> XMHLNPAEKEKLQIFLASELLLRRKARGLKLNYPEAVAIITSFIMEGARDGKTVAMLMEEGKHVLTRDDVMEGVPEMIDDIQAEATFPDGTKLVTVHNPIS;> MSNNNYIVPGEYRVAEGEIEINAGREKTTIRVSNTGDRPIQVGSHIHFVEVNKELLFDRAEGIGRRLNIPSGTAARFEPGEEMEVELTELGGNREVFGISDLTNGSVDNKELILQRAKELGYKGVE;> MKINRQQYAESYGPTVGDEVRLADTDLWIEVEKDYTTYGDEVNFGGGKVLREGMGENGTYTRTENVLDLLLTNALILDYTGIYKADIGVKDGYIVGIGKGGNPDIMDGVTPNMIVGTATEVIAAEGKIVTAGGIDTHVHFINPDQVDVALANGITTLFGGGTGPAEGSKATTVTPGPWNIEKMLKSTEGLPINVGILGKGHGSSIAPIMEQIDAGAAGLKIHEDWGATPASIDRSLTVADEADVQVAIHSDTLNEAGFLEDTLRAINGRVIHSFHVEGAGGGHAPDIMAMAGHPNVLPSSTNPTRPFTVNTIDEHLDMLMVCHHLKQNIPEDVAFADSRIRPETIAAEDILHDLGIISMMSTDALAMGRAGEMVLRTWQTADKMKKQRGPLAEEKNGSDNFRLKRY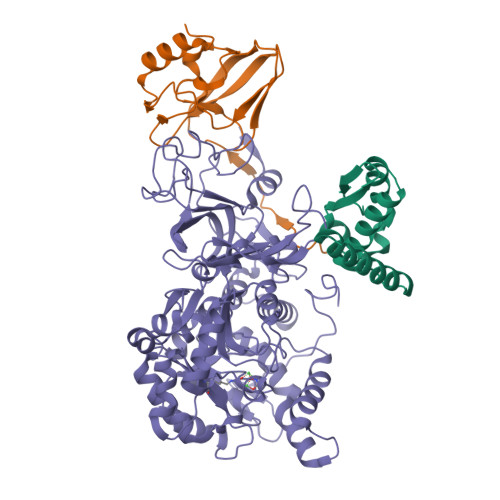VSKYTINPAIAQGIAHEVGSIEEGKFADLVLWEPKFFGVKADRVIKGGIIAYAQIGDPSASIPTPQPVMGRRMYGTVGDLIHDTNITFMSKSSIQQGVPAKLGLKRRIGTVKNCRNIGKKDMKWNDVTTDIDINPETYEVKVDGEVLTCEPVKELPMAQRYFLF> TQVILNCSALPCLLHLLSSPKESIRKEACWTVSNITAGNRAQIQAVIDANIFPVLIEILQKAEFRTRKEAAWAITNATSGGTPEQIRYLVALGCIKPLCDLLTVMDSKIVQVALNGLENILRLGEQES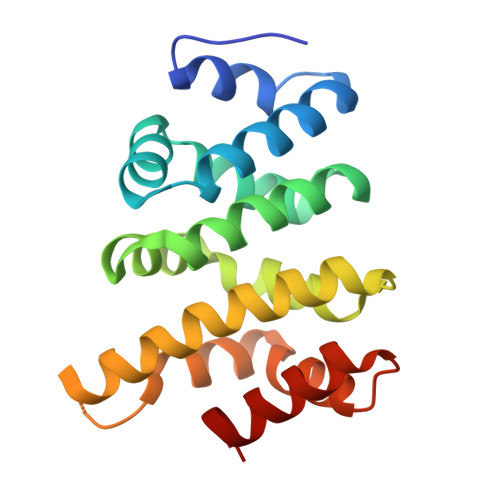KQNGIGINPYCALIEEAYGLDKIEFLQSHENQEIYQKAFDLIEHYFG Botulinum neurotoxins (BoNT) are a group of clostridial toxins that cause the potentially fatal neuroparalytic disease botulism. BoNTs are composed of three domains—a cell-binding domain, a translocation domain, and a catalytic domain. For BoNT/A, the HC/A binds to both a ganglioside (e.g., GD1a) and synaptic vesicle protein 2 (SV2C) at the nerve terminals of the neuromuscular junction. In this paper, we present the crystal structures of the botulinum neurotoxin A2 cell binding domain, both alone and in complex with its receptor ganglioside GD1a at 1.63 and 2.10 Å, respectively.

The structure of HC/A2:GD1a complex was solved by molecular replacement to 2.1 Å with two molecules (A and B) in the asymmetric unit. Clear positive difference map electron density was observed at the GBS of molecule B that could be readily modelled as GD1a, whereas for molecule A, the GBS is inaccessible to GD1a due to crystal packing. Therefore, the HC/A2:GD1a asymmetric unit contains both the GD1a-bound and unbound states of HC/A2. A total of 5/6 monosaccharides are clearly defined by the electron density. GD1a forms a total of 10 hydrogen bonding interactions to HC/A2, two of which are water-mediated. The superimposition of molecule ‘A’ and ‘B’ (for Cα atoms) yields an RMSD of 0.47 Å, indicating that the overall structure of the molecule does not change upon binding GD1a. However, the loop spanning residues 1269–1277 appears to widen upon GD1a binding—the distance between the Cα atoms of residues 1269 and 1277 is ~4.5 Å greater in molecule B than that in molecule A. This change in loop positioning is accompanied by the rotation of Phe 1278 towards the GBS, a feature that has been observed previously in the HC/A3:GD1a, HC/A4:GD1a, and HC/A5:GM1b structures. Using DynDom (which estimates domain motions in proteins), the HCN/A2 subdomain appears to rotate 3.6° in one direction when bound to GD1a, but 6.7° in the other direction when bound to SV2C. In both the HC/A2 and HC/A2:GD1a structures, clear electron density was observed between Lys 1236 and Cys 1280 indicating the presence of an unusual covalent bridge between the two residues.

>MHHHHHHKNIVNTSILSIVYKKDDLIDLSRYGAKINIGDRVYYDSIDKNQIKLINLESSTIEVILKNAIVYNSMYENFSTSFWIKIPKYFSKINLNNEYTIINCIENNSGWKVSLNYGEIIWTLQDNKQNIQRVVFKYSQMVNISDYINRWIFVTITNNRLTKSKIYINGRLIDQKPISNLGNIHASNKIMFKLDGCRDPRRYIMIKYFNLFDKELNEKEIKDLYDSQSNSGILKDFWGNYLQYDKPYYMLNLFDPNKYVDVNNIGIRGYMYLKGPRGSVVTTNIYLNSTLYEGTKFIIKKYASGNEDNIVRNNDRVYINVVVKNKEYRLATNASQAGVEKILSALEIPDVGNLSQVVVMKSKDDQGIRNKCKMNLQDNNGNDIGFIGFHLYDNIAKLVASNWYNRQVGKASRTFGCSWEFIPVDDGWGESSL[2x]> GSHNMAGRSMQAARCPTDELSLSNCAVVSEKDYQSGQHVIVRTSPNHKYIFTLRTHPSVVPGSVAFSLPQRKWAGLSIGQEIEVALYSFDKAKQCIGTMTIEIDFLQKKNIDSNPYDTDKMAAEFI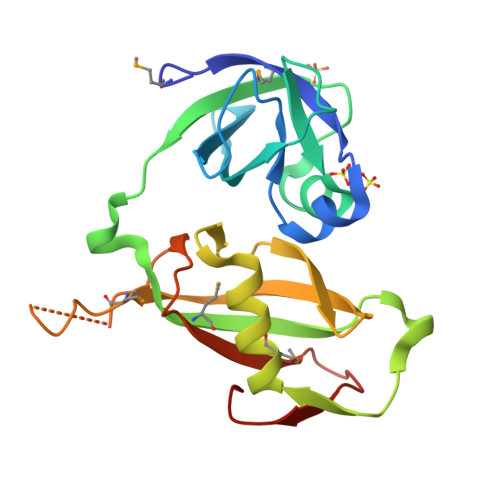QQFNNQAFSVGQQLVFSFNDKLFGLLVKDIEAMDPSILKGEPASGKRQKIEVGLVVGNSQVAFEKAENSSLNLIGKAKTKENRLE> MPDVDWNMLRGNATQAAAGAYVPYSRFAVGAAALVDDGRVVTGCNVENVSYGLTLCAECAVVCALHSTGGGRLLALACVDGHGSVLMPCGR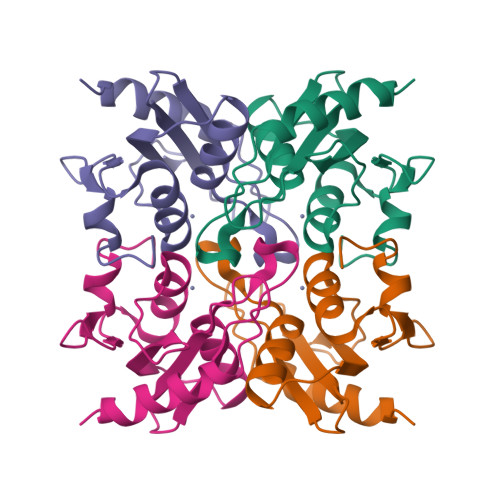CRQVLLEHGGSELLIDHPVRPRRLGDLLPDAFGLDDLPRERR> MGWSLPKEKGLILCLWNKFCRWFHRRESWAQSRDEQNLLQQKRIWESPLLLAAKENNVQALYKLLKFEGCEVHQKGAMGETALHIAALYDNNEAAQVLMEAAPELVFEPMTSELYEGQTALHIAVINQNVNLVRALLARGASVSARATGSVFHYRPHNLIYYGEHPLSFAACVGSEEIVRLLIEHGADIRAQDSLGNTVLHILILQPNKTFACQMYNLLLSYDGGDHLKSLELVPNNQGLTPFKLAGVEGNIVMFQHLMQKRKHIQWTYGPLTSTLYDLTEIDSSGDDQSLLELIVTTKKREARQILDQTPVKELVSLKWKRYGRPYFCVLGAIYVLYIICFTMCCVYRPLKPRITNRTNPRDNTLLQQKLLQEAYVTPKDDLRLVGELVSIVGAVIILLVEIPDIFRLGVTRFFGQTILGGPFHVIIVTYAFMVLVTMVMRLTNSDGEVVPMSFALVLGWCNVMYFARGFQMLGPFTIMIQKMIFGDLMRFCW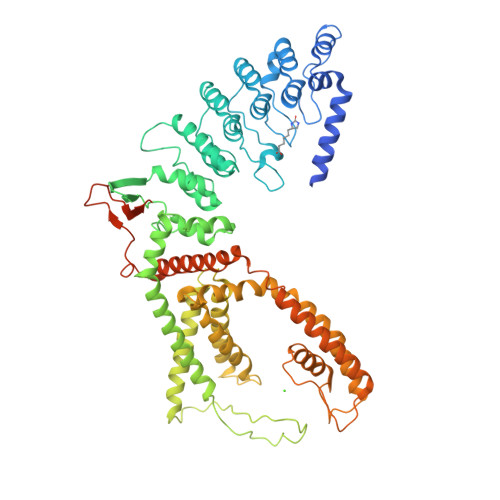LMAVVILGFASAFYIIFQTEDPDELGHFYDYPMALFSTFELFLTIIDGPANYDVDLPFMYSITYAAFAIIATLLMLNLLIAMMGDTHWRVAHERDELWRAQVVATTVMLERKLPRCLWPRSGICGREYGLGDRWFLRVEDRQDLNRQRIRRYAQAFQQQDDLYSEDLEKDSGEKLVPRLVPR> MGLENIRDAVRKFLTGSTPYEKAVDEFIKDLQKSLISSDVNVKLVFSLTAKIKERLNKEKPPSVLERKEWFISIVYDELSKLFGGDKEPNVNPTKLPFIIMLVGVQGSGKTTTAGKLAYFYKKRGYKVGLVAADVYRPAAYDQLLQLGNQIGVQVYGEPNNQNPIEIAKKGVDIFVKNKMDIIIVDTAGRHGYGEETKLLEEMKEMYDVLKPDDVILVIDASIGQKAYDLASRFHQASPIGSVIITKMDGTAKGGGALSAVVATGATIKFIGTGEKIDELETFNAKRFVSRILGMGDIESILEKVKGLEEYDKIQKKMEDVMEGKGKLTLRDVYAQIIALRKMGPLSKVLQHIPGLGIMLPTPSEDQLKIGEEKIRRWLA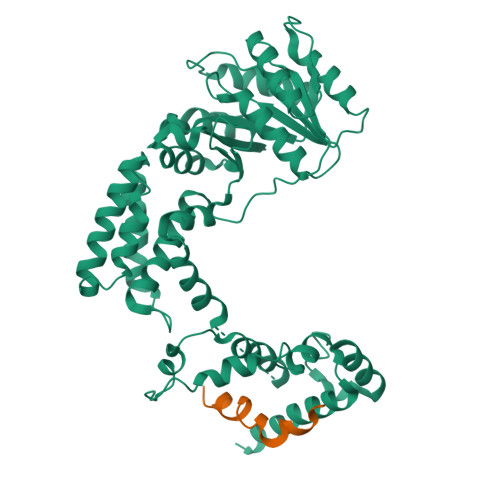ALNSMTYKELENPNIIDKSRMRRIAEGSGLEVEEVRELLEWYNNMNRLLKMVK;> ARSGSGSGSGSKLIRVGIILVLLIWGTVLLLKSIPHHHHHHH1-[(1r,3r)-3-(methylcarbamoyl)cyclobutyl]-N-[(1-methylpiperidin-4-yl)methyl]-2-(3,4,5-trimethoxyphenyl)-1H-1,3-benzimidazole-6-carboxamide | C30 H39 N5 O5 | 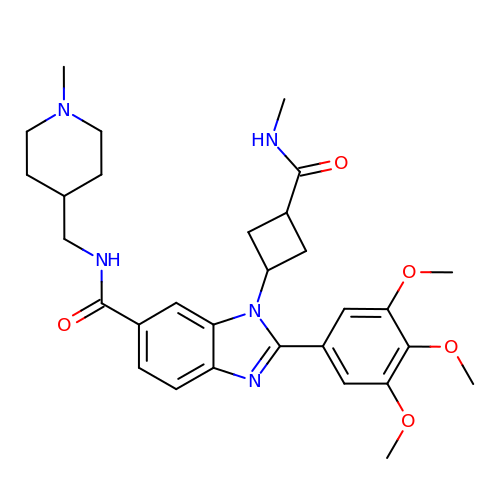UIZVBBVWCDAVED-HZCBDIJESA-N>[2x]GEIRPTIGQQMETGDQRFGDLVFRQLAPNVWQHTSYLDMPGFGAVASNGLIVRDGGRVLVVDTAWTDDQTAQILNWIKQEINLPVALAVVTHAHQDKMGGMDALHAAGIATYANALSNQLAP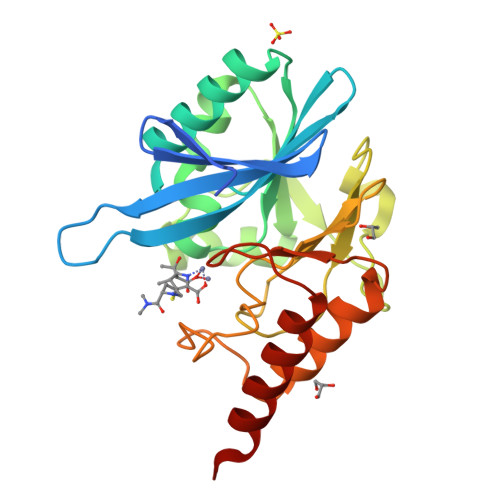QEGMVAAQHSLTFAANGWVEPATAPNFGPLKVFYPGPGHTSDNITVGIDGTDIAFGGCLIKDSKAKSLGNLGDADTEHYAASARAFGAAFPKASMIVMSHSAPDSRAAITHTARMADKLRKLX> QL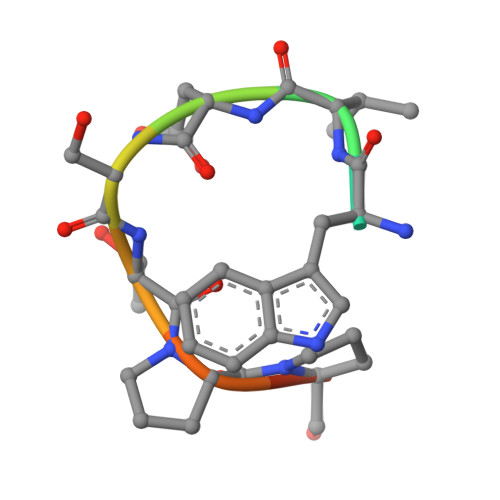WVDSTPPPG> MKAVKSERERGSRRRHRDGDVVLPAGVVVKQERLSPEVAPPAHRRPDHSGGSPSPPTSEPARSGHRGNRARGVSRSPPKKKNKASGRRSKSPRSKRNRSPHHSTVKVKQEREDHPRRGREDRQHREPSEQEHRRARNSDRDRHRGHSHQRRTSNERPGSGQGQGRDRDTQNLQAQEEEREFYNARRREHRQRNDVGGGGSESQELVPRPGGNNKEKEVPAKEKPSFELSGALLEDTNTFRGVVIKYSEPPEARIPKKRWRLYPFKNDEVLPVMYIHRQSAYLLGRHRRIADIPIDHPSCSKQHAVFQYRLVEYTRADGTVGRRVKPYIIDLGSGNGTFLNNKRIEPQRYYELKEKDVLKFGFSSREYVLLHESSDTSEIDRKDDEDEEEEEEVSDS;> MNPLTKVKLINELNEREVQLGVADKVSWHSEYKDSAWIFLGGLPYELTEGDIICVFSQYGEIVNINLVRDKKTGKSKGFCFLCYEDQRSTILAVDNFNGIKIKGRTIRVDHVSNYRAPKDSEEIDDVTRQLQEKGCGARTPSPSLSESSEDEKPTKKHKKDKKEKKKKKKEKEKADREVQAEQPSSSSPRRKTVKEKDDTGPKKHSSKNSERAQKSEPREGQKLPKSRTAYSGGAEDLERELKKEKPKHEHKSSSRREAREEKTRIRDRGRSSDAHSSWYNGRSEGRSYRSRSRSRDKSHRHKRARRSRERESSNPSDRWRH;> METILEQQRRYHEEKERLMDVMAKEMLTKKSTLRDQINSDHRTRAMQDRYMEVSGNLRDLYDDKDGLRKEELNAISGPNEFAEFYNRLKQIKEFHRKHPNEICVPMSVEFEELLKARENPSEEAQNLVEFTDEEGYGRYLDLHDCYLKYINLKASEKLDYITYLSIFDQLFDIPKERKNAEYKRYLEMLLEYLQDYTDRVKPLQDQNELFGKIQAEFEKKWENGTFPGWPKETSSALTHAGAHLDLSAFSSWEELASLGLDRLKSALLALGLKCGGTLEERAQRLFSTKGKSLESLDTSLFAKNPKSKGTKRDTERNKDIAFLEAQIYEYVEILGEQRHLTHENVQRKQARTGEEREEEEEEQISESESEDEENEIIYNPKNLPLGWDGKPIPYWLYKLHGLNINYNCEICGNYTYRGPKAFQRHFAEWRHAHGMRCLGIPNTAHFANVTQIEDAVSLWAKLKLQKASERWQPDTEEEYEDSSGNVVNKKTYEDLKRQGLL;> MGKSDFLTPKAIANRIKSKGLQKLRWYCQMCQKQCRDENGFKCHCMSESHQRQLLLASENPQQFMDYFSEEFRNDFLELLRRRFGTKRVHNNIVYNEYISHREHIHMNATQWETLTDFTKWLGREGLCKVDETPKGWYIQYIDRDPETIRRQLELEKKKKQDLDDEEKTAKFIEEQVRRGLEGKEQEVPTFTELSRENDEEKVTFNLSKGACSSSGATSSKSSTLGPSALKTIGSSASVKRKESSQSSTQSKEKKKKKSALDEIMEIEEEKKRTARTDYWLQPEIIVKIITKKLGEKYHKKKAIVKEVIDKYTAVVKMIDSGDKLKLDQTHLETVIPAPGKRILVLNGGYRGNEGTLESINEKTFSATIVIETGPLKGRRVEGIQYEDISKLA;> MFLYNLTLQRATGISFAIHGNFSGTKQQEIVVSRGKILELLRPDPNTGKVHTLLTVEVFGVIRSLMAFRLTGGTKDYIVVGSDSGRIVILEYQPSKNMFEKIHQETFGKSGCRRIVPGQFLAVDPKGRAVMISAIEKQKLVYILNRDAAARLTISSPLEAHKANTLVYHVVGVDVGFENPMFACLEMDYEEADNDPTGEAAANTQQTLTFYELDLGLNHVVRKYSEPLEEHGNFLITVPGGSDGPSGVLICSENYITYKNFGDQPDIRCPIPRRRNDLDDPERGMIFVCSATHKTKSMFFFLAQTEQGDIFKITLETDEDMVTEIRLKYFDTVPVAAAMCVLKTGFLFVASEFGNHYLYQIAHLGDDDEEPEFSSAMPLEEGDTFFFQPRPLKNLVLVDELDSLSPILFCQIADLANEDTPQLYVACGRGPRSSLRVLRHGLEVSEMAVSELPGNPNAVWTVRRHIEDEFDAYIIVSFVNATLVLSIGETVEEVTDSGFLGTTPTLSCSLLGDDALVQVYPDGIRHIRADKRVNEWKTPGKKTIVKCAVNQRQVVIALTGGELVYFEMDPSGQLNEYTERKEMSADVVCMSLANVPPGEQRSRFLAVGLVDNTVRIISLDPSDCLQPLSMQALPAQPESLCIVEMGGTEKQDELGERGSIGFLYLNIGLQNGVLLRTVLDPVTGDLSDTRTRYLGSRPVKLFRVRMQGQEAVLAMSSRSWLSYSYQSRFHLTPLSYETLEFASGFASEQCPEGIVAISTNTLRILALEKLGAVFNQVAFPLQYTPRKFVIHPESNNLIIIETDHNAYTEATKAQRKQQMAEEMVEAAGEDERELAAEMAAAFLNENLPESIFGAPKAGNGQWASVIRVMNPIQGNTLDLVQLEQNEAAFSVAVCRFSNTGEDWYVLVGVAKDLILNPRSVAGGFVYTYKLVNNGEKLEFLHKTPVEEVPAAIAPFQGRVLIGVGKLLRVYDLGKKKLLRKCENKHIANYISGIQTIGHRVIVSDVQESFIWVRYKRNENQLIIFADDTYPRWVTTASLLDYDTVAGADKFGNICVVRLPPNTNDEVDEDPTGNKALWDRGLLNGASQKAEVIMNYHVGETVLSLQKTTLIPGGSESLVYTTLSGGIGILVPFTSHEDHDFFQHVEMHLRSEHPPLCGRDHLSFRSYYFPVKNVIDGDLCEQFNSMEPNKQKNVSEELDRTPPEVSKKLEDIRTRYAF;> MDFQHRPGGKTGSGGVASSSESNRDRRERLRQLALETIDINKDPYFMKNHLGSYECKLCLTLHNNEGSYLAHTQGKKHQTNLARRAAKEAKEAPAQPAPEKVKVEVKKFVKIGRPGYKVTKQRDSEMGQQSLLFQIDYPEIAEGIMPRHRFMSAYEQRIEPPDRRWQYLLMAAEPYETIAFKVPS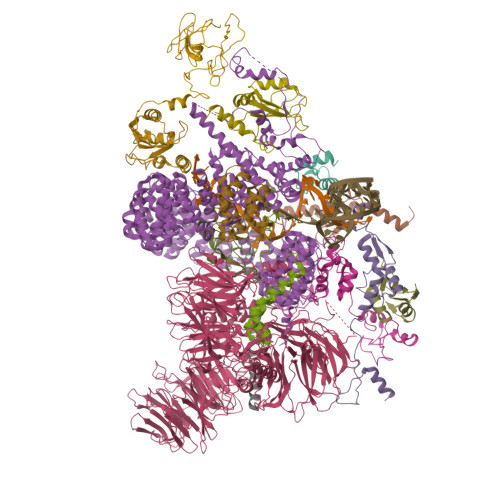REIDKAEGKFWTHWNRETKQFFLQFHFKMEKPPAPPSLPAGPPGVKRPPPPLMNGLPPRPPLPESLPPPPPGGLPLPPMPPTGPAPSGPPGPPQLPPPAPGVHPPAPVVHPPASGVHPPAPGVHPPAPGVHPPAPGVHPPTSGVHPPAPGVHPPAPGVHPPAPGVHPPAPGVHPPAPGVHPPPSAGVHPQAPGVHPAAPAVHPQAPGVHPPAPGMHPQAPGVHPQPPGVHPSAPGVHPQPPGVHPSNPGVHPPTPMPPMLRPPLPSEGPGNIPPPPPTN;> MPRIMIKGGVWRNTEDEILKAAVMKYGKNQWSRIASLLHRKSAKQCKARWYEWLDPSIKKTEWSREEEEKLLHLAKLMPTQWRTIAPIIGRTAAQCLEHYEFLLDKAAQRDNEEETTDDPRKLKPGEIDPNPETKPARPDPIDMDEDELEMLSEARARLANTQGKKAKRKAREKQLEEARRLAALQKRRELRAAGIEIQKKRKRKRGVDYNAEIPFEKKPALGFYDTSEENYQALDADFRKLRQQDLDGELRSEKEGRDRKKDKQHLKRKKESDLPSAILQTSGVSEFTKKRSKLVLPAPQISDAELQEVVKVGQASEIARQTAEESGITNSASSTLLSEYNVTNNSVALRTPRTPASQDRILQEAQNLMALTNVDTPLKGGLNTPLHESDFSGVTPQRQVVQTPNTVLSTPFRTPSNGAEGLTPRSGTTPKPVINSTPGRTPLRDKLNINPEDGMADYSDPSYVKQMERESREHLRLGLLGLPAPKNDFEIVLPENAEKELEEREIDDTYIEDAADVDARKQAIRDAERVKEMKRMHKAVQKDLPRPSEVNETILRPLNVEPPLTDLQKSEELIKKEMITMLHYDLLHHPYEPSGNKKGKTVGFGTNNSEHITYLEHNPYEKFSKEELKKAQDVLVQEMEVVKQGMSHGELSSEAYNQVWEECYSQVLYLPGQSRYTRANLASKKDRIESLEKRLEINRGHMTTEAKRAAKMEKKMKILLGGYQSRAMGLMKQLNDLWDQIEQAHLELRTFEELKKHEDSAIPRRLECLKEDVQRQQEREKELQHRYADLLLEKETLKSKF;> MATEHPEPPKAELQLPPPPPPGHYGAWAAQELQAKLAEIGAPIQGNREELVERLQSYTRQTGIVLNRPVLRGEDGDKAAPPPMSAQLPGIPMPPPPLGLPPLQPPPPPPPPPPGLGLGFPMAHPPNLGPPPPLRVGEPVALSEEERLKLAQQQAALLMQQEERAKQQGDHSLKEHELLEQQKRAAVLLEQERQQEIAKMGTPVPRPPQDMGQIGVRTPLGPRVAAPVGPVGPTPTVLPMGAPVPRPRGPPPPPGDENREMDDPSVGPKIPQALEKILQLKESRQEEMNSQQEEEEMETDARSSLGQSASETEEDTVSVSKKEKNRKRRNRKKKKKPQRVRGVSSESSGDREKDSTRSRGSDSPAADVEIEYVTEEPEIYEPNFIFFKRIFEAFKLTDDVKKEKEKEPEKLDKLENSAAPKKKGFEEEHKDSDDDSSDDEQEKKPEAPKLSKKKLRRMNRFTVAELKQLVARPDVVEMHDVTAQDPKLLVHLKATRNSVPVPRHWCFKRKYLQGKRGIEKPPFELPDFIKRTGIQEMREALQEKEEQKTMKSKMREKVRPKMGKIDIDYQKLHDAFFKWQTKPKLTIHGDLYYEGKEFETRLKEKKPGDLSDELRISLGMPVGPNAHKVPPPWLIAMQRYGPPPSYPNLKIPGLNSPIPESCSFGYHAGGWGKPPVDETGKPLYGDVFGTNAAEFQTKTEEEEIDRTPWGELEPSDEESSEEEEEEESDEDKPDETGFITPADSGLITPGGFSSVPAGMETPELIELRKKKIEEAMDGSETPQLFTVLPEKRTATVGGAMMGSTHIYDMSTVMSRKGPAPELQGVEVALAPEELELDPMAMTQKYEEHVREQQAQVEKEDFSDMVAEHAAKQKQKKRKAQPQDSRGGSKKYKEFKF;> MDAGFFRGTSAEQDNRFSNKQKKLLKQLKFAECLEKKVDMSKVNLEVIKPWITKRVTEILGFEDDVVIEFIFNQLEVKNPDSKMMQINLTGFLNGKNAREFMGELWPLLLSAQENIAGIPSAFLELKKEEIKQRQIEQEKLASMKKQDEDKDKRDKEEKESSREKRERSRSPRRRKSRSPSPRRRSSPVRRERKRSHSRSPRHRTKSRSPSPAPEKKEKTPELPEPSVKVKEPSVQEATSTSDILKVPKPEPIPEPKEPSPEKNSKKEKEKEKTRPRSRSRSKSRSRTRSRSPSHTRPRRRHRSRSRSYSPRRRPSPRRRPSPRRRTPPRRMPPPPRHRRSRSPVRRRRRSSASLSGSSSSSSSSRSRSPPKKPPKRTSSPPRKTRRLSPSASPPRRRHRPSPPATPPPKTRHSPTPQQSNRTRKSRVSVSPGRTSGKVTKHKGTEKRESPSPAPKPRKVELSESEEDKGGKMAAADSVQQRRQYRRQNQQSSSDSGSSSSSEDERPKRSHVKNGEVGRRRRHSPSRSASPSPRKRQKETSPRGRRRRSPSPPPTRRRRSPSPAPPPRRRRTPTPPPRRRTPSPPPRRRSPSPRRYSPPIQRRYSPSPPPKRRTASPPPPPKRRASPSPPPKRRVSHSPPPKQRSSPVTKRRSPSLSSKHRKGSSPSRSTREARSPQPNKRHSPSPRPRAPQTSSSPPPVRRGASSSPQRRQSPSPSTRPIRRVSRTPEPKKIKKAASPSPQSVRRVSSSRSVSGSPEPAAKKPPAPPSPVQSQSPSTNWSPAVPVKKAKSPTPSPSPPRNSDQEGGGKKKKKKKDKKHKKDKKHKKHKKHKKEKAVAAAAAAAVTPAAIAAATTTLAQEEPVAAPEPKKETESEAEDNLDDLEKHLREKALRSMRKAQVSPQS;> MAKIAKTHEDIEAQIREIQGKKAALDEAQGVGLDSTGYYDQEIYGGSDSRFAGYVTSIAATELEDDDDDYSSSTSLLGQKKPGYHAPVALLNDIPQSTEQYDPFAEHRPPKIADREDEYKKHRRTMIISPERLDPFADGGKTPDPKMNARTYMDVMREQHLTKEEREIRQQLAEKAKAGELKVVNGAAASQPPSKRKRRWDQTADQTPGATPKKLSSWDQAETPGHTPSLRWDETPGRAKGSETPGATPGSKIWDPTPSHTPAGAATPGRGDTPGHATPGHGGATSSARKNRWDETPKTERDTPGHGSGWAETPRTDRGGDSIGETPTPGASKRKSRWDETPASQMGGSTPVLTPGKTPIGTPAMNMATPTPGHIMSMTPEQLQAWRWEREIDERNRPLSDEELDAMFPEGYKVLPPPAGYVPIRTPARKLTATPTPLGGMTGFHMQTEDRTMKSVNDQPSGNLPFLKPDDIQYFDKLLVDVDESTLSPEEQKERKIMKLLLKIKNGTPPMRKAALRQITDKAREFGAGPLFNQILPLLMSPTLEDQERHLLVKVIDRILYKLDDLVRPYVHKILVVIEPLLIDEDYYARVEGREIISNLAKAAGLATMISTMRPDIDNMDEYVRNTTARAFAVVASALGIPSLLPFLKAVCKSKKSWQARHTGIKIVQQIAILMGCAILPHLRSLVEIIEHGLVDEQQKVRTISALAIAALAEAATPYGIESFDSVLKPLWKGIRQHRGKGLAAFLKAIGYLIPLMDAEYANYYTREVMLILIREFQSPDEEMKKIVLKVVKQCCGTDGVEANYIKTEILPPFFKHFWQHRMALDRRNYRQLVDTTVELANKVGAAEIISRIVDDLKDEAEQYRKMVMETIEKIMGNLGAADIDHKLEEQLIDGILYAFQEQTTEDSVMLNGFGTVVNALGKRVKPYLPQICGTVLWRLNNKSAKVRQQAADLISRTAVVMKTCQEEKLMGHLGVVLYEYLGEEYPEVLGSILGALKAIVNVIGMHKMTPPIKDLLPRLTPILKNRHEKVQENCIDLVGRIADRGAEYVSAREWMRICFELLELLKAHKKAIRRATVNTFGYIAKAIGPHDVLATLLNNLKVQERQNRVCTTVAIAIVAETCSPFTVLPALMNEYRVPELNVQNGVLKSLSFLFEYIGEMGKDYIYAVTPLLEDALMDRDLVHRQTASAVVQHMSLGVYGFGCEDSLNHLLNYVWPNVFETSPHVIQAVMGALEGLRVAIGPCRMLQYCLQGLFHPARKVRDVYWKIYNSIYIGSQDALIAHYPRIYNDDKNTYIRYELDYIL;> MAAGPISERNQDATVYVGGLDEKVSEPLLWELFLQAGPVVNTHMPKDRVTGQHQGYGFVEFLSEEDADYAIKIMNMIKLYGKPIRVNKASAHNKNLDVGANIFIGNLDPEIDEKLLYDTFSAFGVILQTPKIMRDPDTGNSKGYAFINFASFDASDAAIEAMNGQYLCNRPITVSYAFKKDSKGERHGSAAERLLAAQNPLSQADRPHQLFADAPPPPSAPNPVVSSLGSGLPPPGMPPPGSFPPPVPPPGALPPGIPPAMPPPPMPPGAAGHGPPSAGTPGAGHPGHGHSHPHPFPPGGMPHPGMSQMQLAHHGPHGLGHPHAGPPGSGGQPPPRPPPGMPHPGPPPMGMPPRGPPFGSPMGHPGPMPPHGMRGPPPLMPPHGYTGPPRPPPYGYQRGPLPPPRPTPRPPVPPRGPLRGPLPQ;> MTDRYTIHSQLEHLQSKYIGTGHADTTKWEWLVNQHRDSYCSYMGHFDLLNYFAIAENESKARVRFNLMEKMLQPCGPPADKPEEN;> MAKHHPDLIFCRKQAGVAIGRLCEKCDGKCVICDSYVRPCTLVRICDECNYGSYQGRCVICGGPGVSDAYYCKECTIQEKDRDGCPKIVNLGSSKTDLFYERKKYGFKKR;> MAMQAAKRANIRLPPEVNRILYIRNLPYKITAEEMYDIFGKYGPIRQIRVGNTPETRGTAYVVYEDIFDAKNACDHLSGFNVCNRYLVVLYYNANRAFQKMDTKKKEEQLKLLKEKYGINTDPPK>[2x]MEGAKPTLQLVYQAVQALYHDPDPSGKERASFWLGELQRSVHAWEISDQLLQIRQDVESCYFAAQTMKMKIQTSFYEL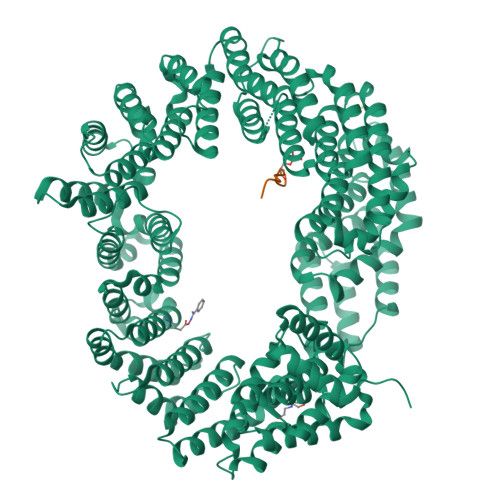PTDSHASLRDSLLTHIQNLKDLSPVIVTQLALAIADLALQMPSWKGCVQTLVEKYSNDVTSLPFLLEILTVLPEEVHSRSLRIGANRRTEIIEDLAFYSSTVVSLLMTCVEKAGTDEKMLMKVFRCLGSWFNLGVLDSNFMANNKLLALLFEVLQQDKTSSNLHEAASDCVCSALYAIENVETNLPLAMQLFQGVLTLETAYHMAVAREDLDKVLNYCRIFTELCETFLEKIVCTPGQGLGDLRTLELLLICAGHPQYEVVEISFNFWYRLGEHLYKTNDEVIHGIFKAYIQRLLHALARHCQLEPDHEGVPEETDDFGEFRMRVSDLVKDLIFLIGSMECFAQLYSTLKEGNPPWEVTEAVLFIMAAIAKSVDPENNPTLVEVLEGVVRLPETVHTAVRYTSIELVGEMSEVVDRNPQFLDPVLGYLMKGLCEKPLASAAAKAIHNICSVCRDHMAQHFNGLLEIARSLDSFLLSPEAAVGLLKGTALVLARLPLDKITECLSELCSVQVMALKKLLSQEPSNGISSDPTVFLDRLAVIFRHTNPIVENGQTHPCQKVIQEIWPVLSETLNKHRADNRIVERCCRCLRFAVRCVGKGSAALLQPLVTQMVNVYHVHQHSCFLYLGSILVDEYGMEEGCRQGLLDMLQALCIPTFQLLEQQNGLQNHPDTVDDLFRLATRFIQRSPVTLLRSQVVIPILQWAIASTTLDHRDANCSVMRFLRDLIHTGVANDHEEDFELRKELIGQVMNQLGQQLVSQLLHTCCFCLPPYTLPDVAEVLWEIMQVDRPTFCRWLENSLKGLPKETTVGAVTVTHKQLTDFHKQVTSAEECKQVCWALRDFTRLFR;>ESKSYGSGSRRERSRERDHSRSREKSRRHKSRSRDRHDDYYRERSRERERHRDRDRDRDRERDREREYRH[2x]>[4x]MRGSHHHHHHENLYFQGSPRWILGDKFDTVFPHKGSLKVLWESRWKFACSKSVYPFHDGSIEDFEPIFNHLISKNINDAASDEYTQAFLPTASALEEKAAQALQAGKHEEASNLLCRAAVVYRISRFPYVDITKPNSIKRVAFERQKQAYLKATSLWTQPIREVTVPHTYRTGNDGAHIPIYIRTPAGADQSNPVPIVLIMTGLDGYRPDNSQRTHEILARGWAAVVAEIPGTADCPADPADPASPDRLWDSVLSYLDQRPELNTAKMVVWGLSAGGYYAIRAAHTHRDRLLGAIAHGPGCHYYLDPEWLAKVNDHEYPFEITAAWATKHGYKTVEEFVAGAQKKFSLVETGIVDQPSCRLLLLNGVDDGVVPIEDCLVLFEHGSPKEGRFYKGLPHMGYPNSLPVSYEWLEQVLASPSKTKN

A common step during their assembly is polyketide trimming, which Afyg1p, Wdyg1p, and PlAntI catalyze. In summary, the N‐ and C‐domains in all three enzymes are oriented in a back‐to‐back fashion forming an interface that encloses the intramolecular binding cavity next to the active site. The catalytic triad is formed exclusively by the α/β‐hydrolase domain with the nucleophilic serine located in the consensus GXSXG esterase motif. The resulting Ser‐His‐Asp network is perfectly aligned with distances in the range of 2.5–2.8 Å between the active‐site residues.

For example, in Aspergillus fumigatus (Af), the type I PKS AfPksP produces the naphthopyrone heptaketide YWA1, whose acetoacetyl side chain is removed by the serine hydrolase Afyg1p. The specificity pocket of Afyg1p and Wdyg1p share many conserved residues and molecule‐binding features with some notable differences. The electron density map displays the pi‐stacking of the planar naphthalene ring systems with Met381 and Tyr37 (analogous to Met379 and Tyr39, respectively, of Wdyg1p). Here, the hydroxyl groups of the surrogate are oriented toward the active site of Afyg1p but form only loose H─bonding interactions with Ser257Oγ and His380Nε (3.7 and 3.9 Å). Co‐crystallization experiments of the Afyg1pS257A mutant with 1,3‐DHN support these minor interactions with the active site since the ligand binds identically without the nucleophilic hydroxyl group of Ser257. In contrast to Wdyg1p, the cavity in Afyg1p:1,3‐DHN is enclosed by Tyr383, which is rotated by 90° compared to the apo state and extends additional pi–pi‐stacking interactions with 1,3‐DHN (3.7 Å). Strikingly, in comparison with the Afyg1p:1,3‐DHN complex structure, THN is rotated 90° in‐plane and shifted almost 4 Å deeper into the pocket, resulting in an open and spacious binding cavity between the active site and the surrounding bulk solvent that extends ≈7 × 10 × 12 Å3.>PSVYDAAAQLTADVKKDLRDSWKVIGSDKKGNGVAVMTTLFADNQETIGYFKRLGDVSQGMANDKLRGHSITLMYALQNFIDQLDNPDDLVCVVEKFAVNHITRKISAAEFGKINGPIKKVLASKNFGDKYANAWAKLVAVVQAAL[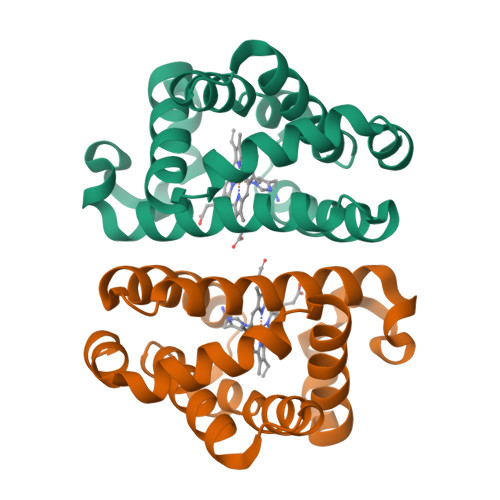2x]> MSRKKNPSVIQFEKAITEKNYEAACTELLDILNKIDTNFGDIEGIDFDYPQQLETLMQDRIVYFCTRMSNAITQLFCDPQFSLSESGANRFFVVQRWLNLIFASSPYINADHILQTYNCNPERDSIYDIYLEPNKNVLMKFAVLYLPESNVNLNLDTMWETDKNICGSLCFALQSPRFIGTPAAFSKRSTILQWFPAKLEQFHVLDDLPSNISHDVYMHCSYDTAENKHNVKKALNQVIRSHLLKCGWQDRQITQIGMRNGKPVMVVVLEHFHSSHSIYRTHSTSMIAAREQFYLIGLGNNAVDQAGRDVFDEFHEFDGSNILKKLAFLKEMCEKNDAAVLYMPSIGMDLATIFVSNARFAPIQVIALGHPATTHSEFIEYVIVEDDYVGSESCFSETLLRLPKDALPYVPSSLAPTDVQYVLRETPEVVNIGIAATTMKLNPYFLETLKTI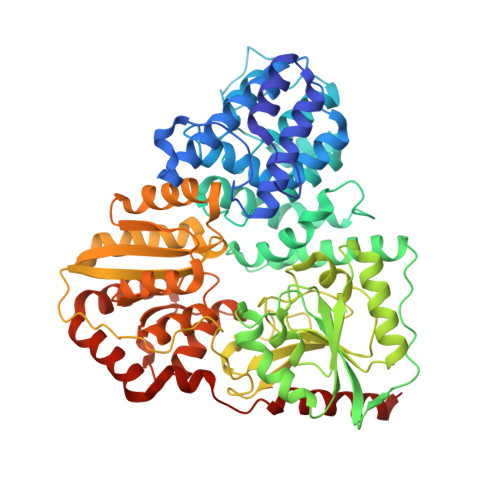RDRAKVKVHFHFALGQSIGITHPYVARFIRSYLGDDATAHPHSPYNRYLDILHNCDMMLNPFPFGNTNGIIDMVTLGLVGVCKTGPEVHEHIDEGLFKRLGLPEWLIADSVEDYIERAIRLAENHQERLALRRHIIENNGLKTLFSGDPSPMGKTLFAKLTEWRQTNGI> MSDTWSSIQAHKKQLDSLRERLQRRRKQDSGHLDLRNPEAALSPTFRSDSPVPTAPTSGGPKPSTASAVPELATDPELEKKLLHHLSDLALTLPTDAVSICLAISTPDAPATQDGVESLLQKFAAQELIEVKRGLLQDDAHPTLVTYADHSKLSAMMGAVAEKKG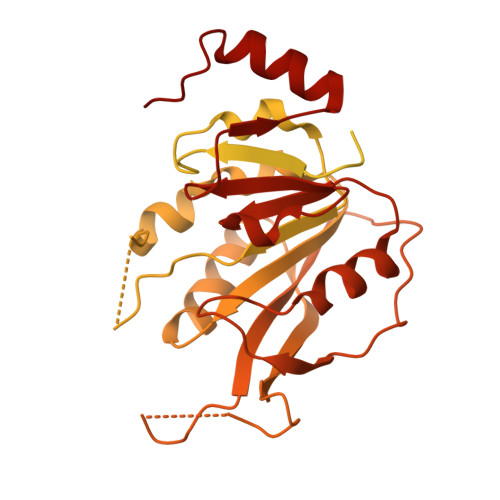PGEVAGTVTGQKRRAEQDSTTVAAFASSLVSGLNSSASEPAKEPAKKSRKHAASDVDLEIESLLNQQSTKEQQSKKVSQEILELLNTTTAKEQSIVEKFRSRGRAQVQEFCDYGTKEECMKASDADRPCRKLHFRRIINKHTDESLGDCSFLNTCFHMDTCKYVHYEIDACMDSEAPGSKDHTPSQELALTQSVGGDSSADRLFPPQWICCDIRYLDVSILGKFAVVMADPPWDIHMELPYGTLTDDEMRRLNIPVLQDDGFLFLWVTGRAMELGRECLNLWGYERVDEIIWVKTNQLQRIIRTGRTGHWLNHGKEHCLVGVKGNPQGFNQGLDCDVIVAEVRSTSHKPDEIYGMIERLSPGTRKIELFGRPHNVQPNWITLGNQLDGIHLLDPDVVARFKQRYPDGIISKPKNL> MEPNEGVQLFSAFPPPPPYYKLFTRENIEKVISNMEKEAKHEDDANTLQPK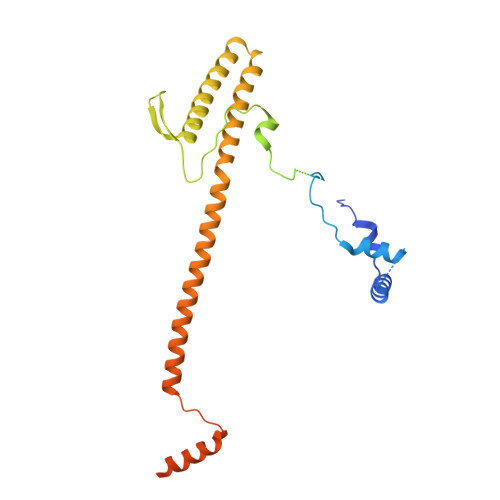TEEEIESLAKLFKKPSCLTSGTYQMFGDTWRLDEAIPSLKEFGIPELYKDIKDGEDEIEVVEYDPKSNAIVGTSFTRVHDYDKNSPIENEKILEDDQHTAMKEKDNESDKTMKDVEEKTEPSLKKEEEDIQMKEPLDSQDTGAVSASSVNEGFRADQKSKDGETSDLIKIPRRAYELRFLSRSLMLNFLELLGIMAKAPEQFPSKVENIRVLLLNLHHLINDYRPHQSRESLIMLLEKQLKHEESQVELLRTHNRQMTETLEKYKSLDFNMEKEGDVIQQLKSSIKKPLSGAEDEQKSRSMFSKNDEKLKKSLELMEDVIKRDLS> SQTIALLNIYRNPQNSSQSADGLR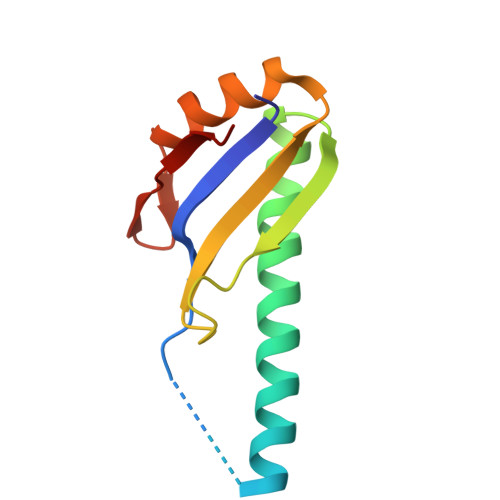SAVSDVEMQEHYDEFFEEVFTEMEEKYGEVEEMNVCDNLGDHLVGNVYVKFRREEDAEKAVIDLNNRWFNGQPIHAELSP Human Shieldin consists of four subunits, REV7 (also known as MAD2L2 or MAD2B, 211 residues), SHLD1 (205 residues), SHLD2 (835 residues), and SHLD3 (250 residues). As the first identified member of the Shieldin complex, REV7 is composed entirely of a HORMA domain, acting as an interaction module in a broad array of cellular pathways. The Shieldin complex acts as the key downstream effector of 53BP1; it not only binds and shields single-stranded DNA ends but also mediates CST- and Polα-dependent fill-ins of DNA breaks. TRIP13 forms a hexamer to drive the REV7-mediated disassembly of Shieldin in an adenosine triphosphate (ATP)-dependent manner, thereby releasing the DSB DNA ends for resection to promote HDR.

We prepared a TRIP13 catalytic mutant (E253Q) that can bind ATP/ATPγS to form a stable hexameric topology but lacks its ATP hydrolysis activity as previously reported. By contrast, monomer F is in the apo-state lacking bound ATPγS, leading to the separation of its large and small AAA+ domains, thereby creating a seam in the hexameric ring of TRIP13. We observe that the N terminus (residues 8 to 14, designated REV7NT) of C-REV7, which was not visible in the crystal structure in the absence of TRIP13, becomes ordered in our cryo-EM structure of the SHLD2.3–REV74–TRIP13 complex and is threaded through the central pore of TRIP13. In this configuration, the highly conserved TRIP13 Trp-221 and Phe-222 of pore loop 1 of monomers B to E, as well as Pro-270 of pore loop 2 of monomers B to D embrace residues 8 to 14 of REV7NT in a ratcheted manner. The structure of the SHLD2.3–REV74–TRIP13 complex reveals two direct intermolecular contact surfaces between SHLD2.3–REV74 and TRIP13 components. The primary interface (site-1) involves contacts between the safety-belt segment of C-REV7 and the conserved and negatively charged loop (110-ENLEEETENII-120; hereafter designated the poly-E loop) of TRIP13 monomer B. The second contact (site-2) forms mainly between the loop 88 to 95 of O-REV7′ and the NTD of TRIP13 monomer E.

>[6x]SDEAVGDLKQALPCVAESPTVHVEVHQRGSSTAKKEDINLSVRKLLNRHNIVFGDYTWTEFDEPFLTRNVQSVSIIDTELKVKDSQPIDLSACTVALHIFQLNEDGPSSENLEEETENIIAANHWVLPAAEFHGLWDSLVYDVEVKSHLLDYVMTTLLFSDKNVNSNLITWNRVVLLHGPPGTGKTSLCKALAQKLTIRLSSRYRYGQLIEINSHSLFSKWFSESGKLVTKMFQKIQDLIDDKDALVFVLIDQVESLTAARNACRAGTEPSDAIRVVNAVLTQIDQIKRHSNVVILTTSNITEKIDVAFVDRADIKQYIGPPSAAAIFKIYLSCLEELMKCQIIYPRQQLLTLRELEMIGFIENNVSKLSLLLNDISRKSEGLSGRVLRKLPFLAHALYVQAPTVTIEGFLQALSLAVDKQFEERKKLAAYI;>STTLTRQDLNFGQVVADVLCEFLEVAVHLILYVREVYPVGIFQKRKKYNVPVQMSCHPELNQYIQDTLHCVKPLLEKNDVEKVVVVILDKEHRPVEKFVFEITQPPLLSISSDSLLSHVEQLLRAFILKISVCDAVLDHNPPGCTFTVLVHTREAATRNMEKIQVIKDFPWILADEQDVHMHDPRLIPLKTMTSDILKMQLYVEERAHKGS[4x];>[2x]MSQVHIFWGAPIAPLKGSGSGSGSGSGSGSGSTTEVILHYRPCESDPTQLPKIAEKAIQDFPTRPLSRFIPWFPYDGSKLPLRPKRSPPASREEIMATL> SMDRRFYGKIVIKGKIKAVTGLHIGSQR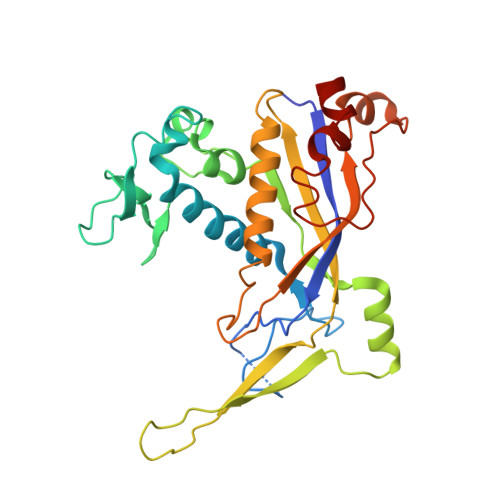DISEIGGIANPVIKDPHTGLPYIPGSSLKGRLRSLFEILVNSRLGEWREKYPSLANYSPGSCRPDNQENCGKFFNRKINRGWIHVCPDYETALACPVCRLFGASGKESNFPSRIIVRDAFLTKEWEEKWRAGEAITEAKIEVGIDRVTSQANPRTNERVVAGAEFEFEIIYNVENTTHWRDDIKNLLTAMALLEDSYLGGSGSRGYGKVKFIFDSFEFRPLDYYRTGKDEDIVSIDAREKSVSDILSGFDSLFSEVEGKLEAG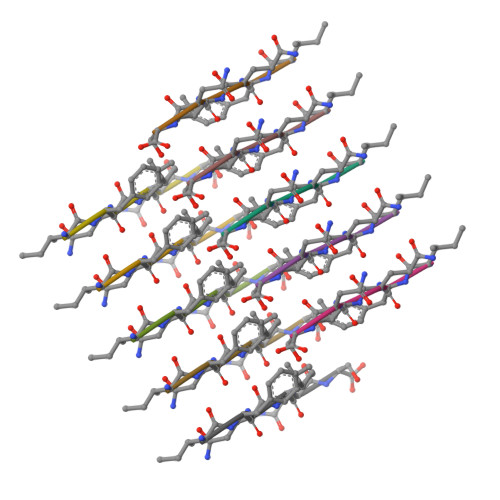> IFQINS>[2x]GAMAKVQVNNVVVLDNPSPFYN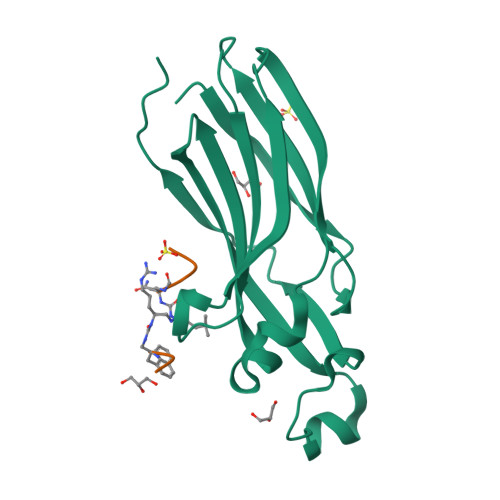PFQFEITFECIEDLSEDLEWKIIYVGSAESEEYDQVLDSVLVGPVPAGRHMFVFQADAPNPGLIPDADAVGVTVVLITCTYRGQEFIRVGYYVNNEYTETELRENPPVKPDFSKLQRNILASNPRVTRFHINWEDN> MLTRNPIVPENHVSNPIVDYEFNQDQSCLIVSTPKSFDIYNVHPLKRIMSQEMPDAGTIRMLHRTNYIAFVSTKKELLHIWDDVKKQDITRVKLDAAVKDLFLSREFIVVSQGDVISIFKFGNPWNKITEDIKFGGVCEFANGLLVYSNEFNLGQIHVTRLQTDAEQVVGKGVLVKAHANPVKMVRLN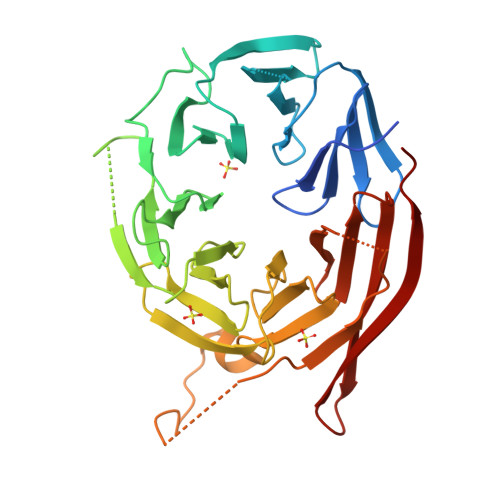RKGDMVATCSQDGTLIRVFQTDNGVLVREFRRGLDRTSIIDMRWSPDGSKLAVVSDKWTLHVFEVFNDAENKRHVLKDWINIKYFQSEWSICNFKLKVSKGSNDCKIAWISDTGLVIVWPNRRLADTFKLNYNDDEHVWWLQLNQRNEIPL3-[3-[2-aminocarbonyl-6-(trifluoromethyloxy)indol-1-yl]phenyl]propanoic acid | C19 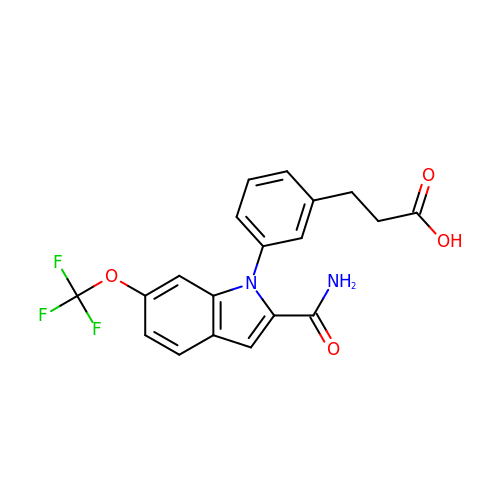H15 F3 N2 O4 | YOCROJNDVYFOIL-UHFFFAOYSA-N> KPQVTILATGGTIAGSAGAVTVDKLLAAVPAINDLATIKGEQISSIGSQEMTGKVWLKLAKRVNELLAQKETEAVIITHGTDTMEETAFFLNLTVKSQKPVVLVGAMRPGSSMSADGPMNLYNAVNVAINKASTNKGVVIVMNDEIHAAREATKLNTTAVNAFASPNTGKIGTVYY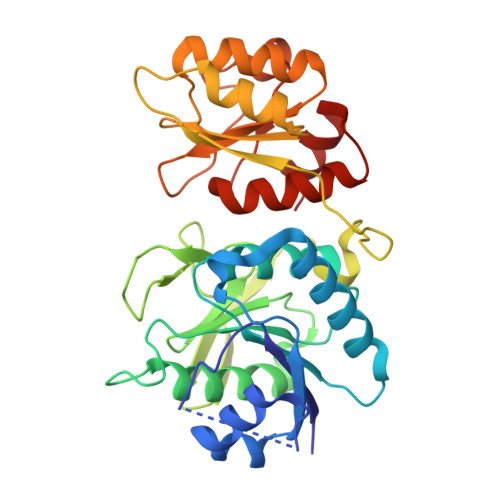GKVEYFTQSVRPHTLASEFDISKIEELPRVDILYAHPDDTDVLVNAALQAGAKGIIHAGMGNGNPFPLTQNALEKAAKSGVVVARSSRVGSGSTTQEAEVDDKKLGFVATESLNPQKARVLLMLALTKTSDREAIQKIFSTY> VNQSETEIEILAEKIARWARARSAEIERDRRLPDELVTRLREAGLLRATMPREVAAPELAPGRALRCAEAVARGDASAGWCVSIAITSALLVAYLPARSREEMFGGGRGVAAGVWAPRGTARSVDGGVVVSGRWPFCSGINHADIMFAGCFVDDRQVPSVVALNKDELQVLDTWHT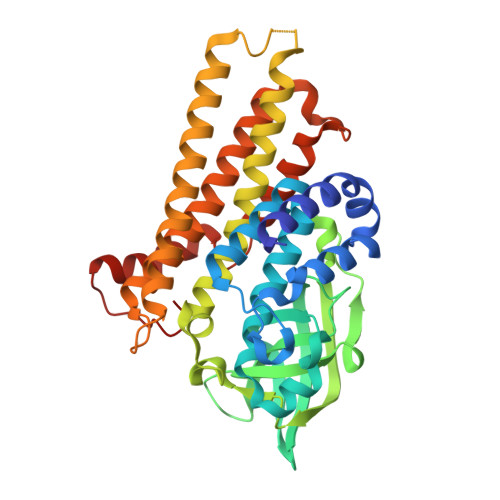LGLRGTGSHDCVADDVFVPADRVFSVFDGPIVDRPLYRFPVFGFFALSIGAAALGNARAAIDDLVELAGGKKGLGSTRTLAERSATQAAAATAESALGAARALFYEVIEAAWQVSHDAEAVPVTMRNRLRLAATHAVRTSADVVRSMYDLAGGTAIYDNAPLQRRFRDAFTATAHFQVNEASRELPGRVLLDQPADVSML[(2~{S},3~{S},4~{E},6~{S},7~{R},10~{R})-3,7-dimethyl-2-[(2~{E},4~{E},6~{R})-6-methyl-6-oxidanyl-7-[(2~{R},3~{R})-3-[(2~{R},3~{S})-3-oxidanylpentan-2-yl]oxiran-2-yl]hepta-2,4-dien-2-yl]-7,10-bis(oxidanyl)-12-oxidanylidene-1-oxacyclododec-4-en-6-yl] 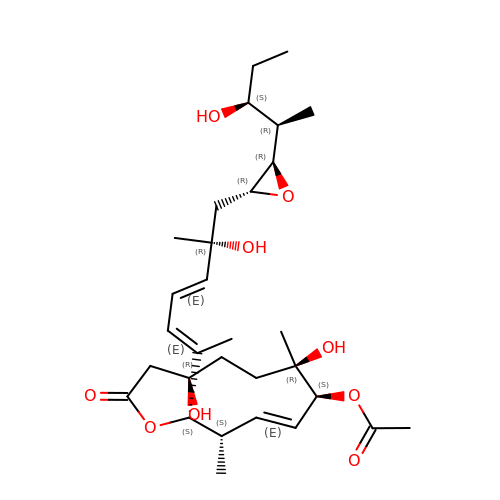ethanoate | C30 H48 O9 | SDUSVHUQNWGNCQ-MLQHUJDKSA-N> GSHMPALPIDQEFDCERFRA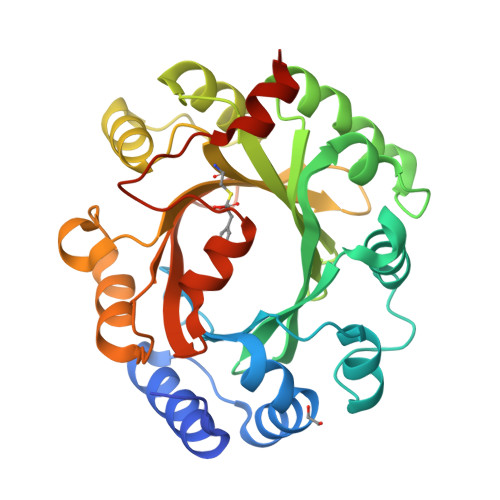DIRATAAAIGAPIAHRLTDTVLEAFRDNFAQGATLWKTTSQPGDQLSYSFFSRLKMDTVSRAIDAGLLDAAHPTLAVVDAWSSLYGGAPVQSGDFDAGRGMAKTWLYFGGLRPAEDILTVPALPASVQARLKDFLALGLAHVRFAAVDWRHHSANVYFRGKGPLDTVQFARIHALSGSTPPAAHVVEEVLAYMPEDYCVAITLDLHSGDIERVCFYALKVPKNALPRIPTRIARFLEVAPSHDVEECNVIGWSFGRSGDYVKAERSYTGNMAEILAGWNCFFHGEEGRDHDLRALHQHTESTMGGAR> MEP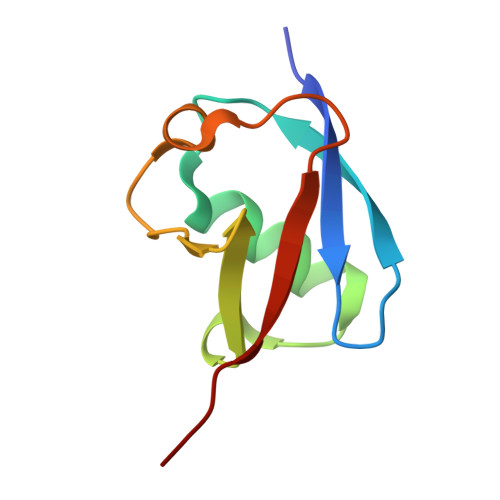LSILVRNNKGRSSTYEVRLTQTVAHLKQQVSGLEGVQDDLFWLTFEGKPLEDQLPLGEYGLKPLSTVFMNLRLRG> HHHHHHMPSGGVFSGSVNLKHVKLGYQYLVNHFLTLLLVPVMAATALELARLGPGELLSLWRSLELDLVHILCSAFLVVFVGTVYVMSRPRPVYLVDYACYKPPASCRVPFATFMEHTRLISDDDKSVRFQTRILERSGLGEDTCLPPANHYIPPNPSMEASRAEAQLVIFSAIDDLVRRTGLKPKDIDILVVNCSLFSPTPSLSAMIINK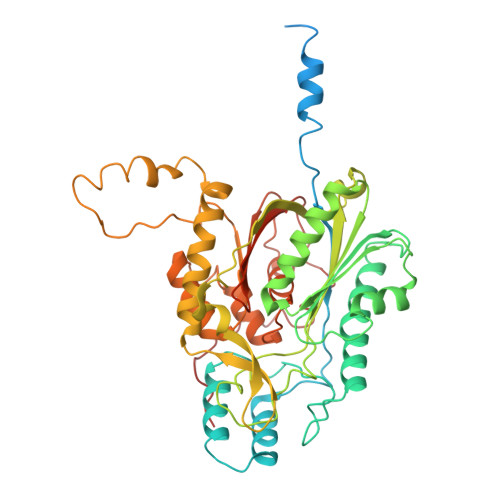YKLRSNIRSFNLSGMGASAGLISIDLARDMLQVHPNSNALVVSTEIITPNFYQGSRRDMLLPNCLFRMGAAAILLSNRRREARRAKYRLVHVVRTHKGADDRAYRCVYEEEDEQGFSGISLSKELMAIAGDALKSNITTIGPLVLPMSEQLLFFFRLVGRKLVNKGWRPYIPDFKLAFEHFCIHAGGRAVIDELQKNLQLSPRHVEASRMTLHRFGNTSSSSLWYELAYIEAKGRMRRGDRVWQIGFGSGFKCNSAVWKCLRSIKTPTNGPWDDCIHRYPVDVPEVVKL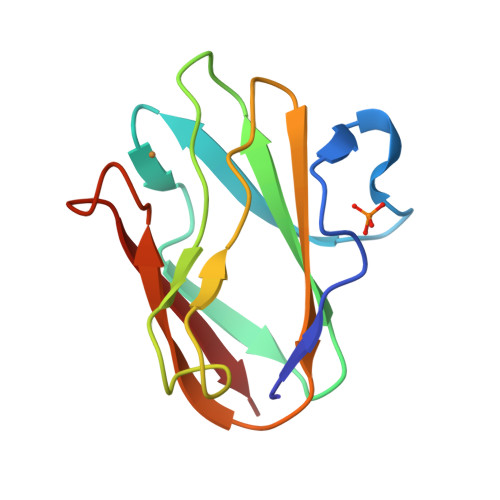> DKATIPSESPFAAAEVADGAIVVDIAKMKYETPELHVKVGDTVTWINREAMPHNVHFVAGVLGEAALKGPMMKKEQAYSLTFTEAGTYDYHCTPHPFARGKVVVE PARA-BROMOBENZYL ALCOHOL 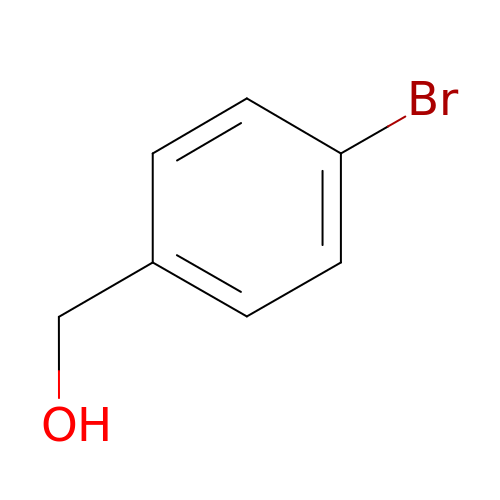| C7 H7 Br O | VEDDBHYQWFOITD-UHFFFAOYSA-N>[2x]GSPGISGGGGGILDSMGRLENLGRIQFSVGYNFQESTLTVKVMKAQELPAKDFSGTSDPFVKIYLLPDKKHKLETKVKRKNLNPHWNETFLFEGFPYEKVVQRILYLQVLDYDRFSRNDPIGEVSIPLNKVDLTQMQTFWKDLKPCSDGSGSRGELLLSLCYNPSANSIIVNIIKARNLKAMDIGGTSDPYVKVWLMYKDKRVEKKKTVTKKRNLNPIFNESFAFDIPTEKLRETTIIITVM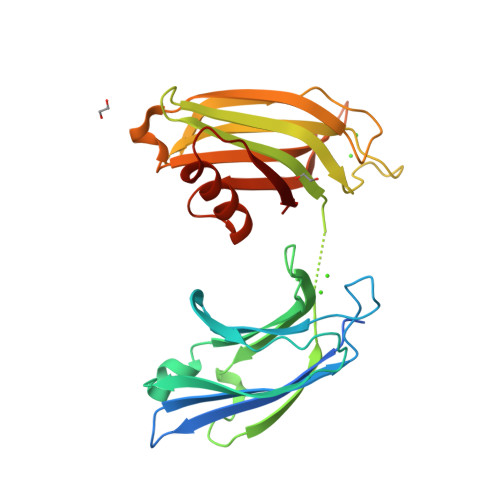DKDKLSRNDVIGKIYLSWKSGPGEVKHWKDMIARPRQPVAQWHQLKA1-(4-thiophen-2-ylphenyl)methanamine 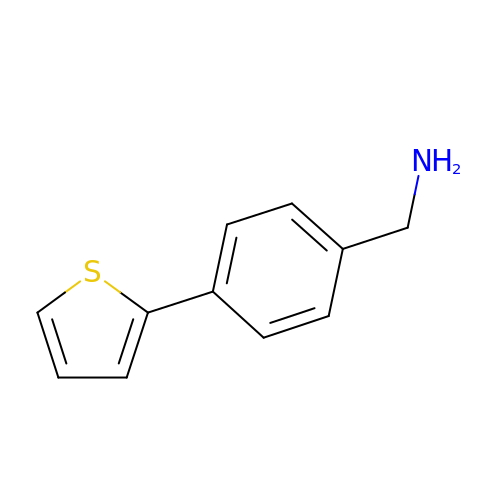| C11 H11 N S | YKNLMMDEWQZCLJ-UHFFFAOYSA-N> MGSSEDQAYRLLNDYANGFMVSQVLFAACELGVFDLLAEAPGPLDVAAVAAGVRASAHGTELLLD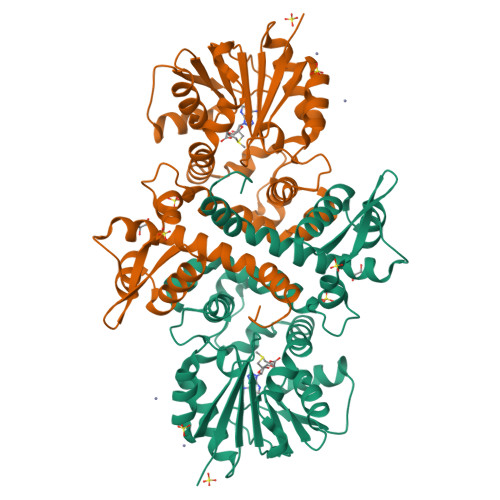ICVSLKLLKVETRGGKAFYRNTELSSDYLTTVSPTSQCSMLKYMGRTSYRCWGHLADAVREGRNQYLETFGVPAEELFTAIYRSEGERLQFMQALQEVWSVNGRSVLTAFDLSVFPLMCDLGGGAGALAKECMSLYPGCKITVFDIPEVVWTAKQHFSFQEEEQIDFQEGDFFKDPLPEADLYILARVLHDWADGKCSHLLERIYHTCKPGGGILVIESLLDEDRRGPLLTQLYSLNMLVQTEGQERTPTHYHMLLSSAGFRDFQFKKTGAIYDAILARKGTHHHHHH>ASRYLTDMTLEEMSRDWFMLMPKQKVAGSLCIKMDQAIMDKTIILKANFSVIFDRLETLILLRAFTEEGAIVGEISPLPSLPGHTGEDVKNAIGVLIGGLEANDNTVRVTETIQRFAWRNSDEDGR[2x];>GSKEDSVEAVGAQLKVYHQQYQDKSREYDQLYEEYTRTSQELQMKRTAIEAFNETIKIFEEQGQTQEKCSKEYLERFRREGNEKEMQRILLNSERLKSRIAEIHESRTKLEQQLRAQASDNREIDKRMNSLKPDLMQLRKIRDQYLVWLTQKGARQKKINEWLGI[2x]

NS1 of an influenza virus is a multifunctional virulence factor that antagonizes the host’s innate immune response and is associated with many strain-specific functions in viral replication and host range. Especially, many mutations occur in the effector domain (ED) of NS1 that interacts with a number of host factors, including retinoic acid-inducible gene 1 (RIG-I), tripartite motif containing 25 (TRIM25), and phosphoinositide 3-kinase (PI3K), during the infection cycle. To this end, we selected four NS1s of human IAV strains that emerged between 1918 and 2004: 1918 H1N1, Puerto Rico 8 (PR8) H1N1, Udorn (Ud) H3N2, and Vietnam (VN) H5N1. Although functionally near-neutral, strain-specific NS1 mutations exhibit long-range epistatic interactions with residues at the p85β-binding interface.

To reveal the mechanistic bases of long-range epistasis and how strain-specific mutations reshaped the energy landscape of NS1 during evolution, we first examined the structure of the NS1:p85β complexes. The structure of the NS1:p85β complex was available for 1918 and PR8 NS1s23,35, and we determined a new crystal structure of VN NS1 bound to p85β in this study. Interestingly, the conformations of NS1s in the complexes were almost identical, with RMSD < 0.5 Å. Although the complex structure of Ud NS1 is not available, it is reasonable to assume that it has a structure similar to other NS1s, considering the sequence identity in the binding interface. This result indicated that the complex structure is not responsible for strain-specific mutational effects on NS1. Given the structural invariance of the complexes, we hypothesized that the structure and dynamics of NS1 in the unbound state are most likely responsible for the strain-specific epistasis and thermodynamic signature for binding. However, there was no difference in the binding among the later strains of 1918 IAV; namely, PR8, Ud, and VN NS1s shared virtually identical binding (kon) and unbinding (koff) rate constants. Notably, the kon value was highly similar in all four NS1s, including 1918 NS1, showing that strain-specific mutations across the NS1s have a near-neutral effect on the p85β-binding rate constant. Indeed, PR8 and VN NS1s underwent the BI-BC dynamics on a sub-ms timescale. The analysis of slow-exchanging residues on the NMR timescale revealed that the population of the BC-like conformer was ~99% for PR8 and VN NS1s and ~90% for 1918 NS1. Overall, core interface residues showed positive epistatic interactions with strain-specific mutations between 1918 and 1972, indicating that the binding interface mutations have less deleterious effects on kon values of NS1s of later IAV strains. This trend reversed between 1972 and 2004, with large negative epistasis.>[4x]MSAI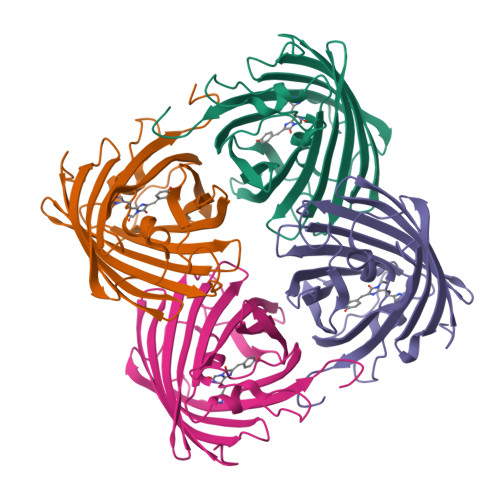KPDMKIKLRMEGNVNGHHFVIDGDGTGKPFEGKQSMDLEVKEGGPLPFAFDILTTAFHYGNRVFAKYPDNIQDYFKQSFPKGYSWERSLTFEDGGICIARNDITMEGDTFYNKVRFYGTNFPANGPVMQKKTLKWEPSTEKMYVRDGVLTGDIHMALLLEGNAHYRCDFRTTYKAKEKGVKLPGYHFVDHCIEILSHDKDYNKVKLYEHAVAHSGLPDNARR N-[([1,1'-biphenyl]-4-yl)sulfonyl]-N-({1-[3,4,6-tri-O-acetyl-2-(acetylamino)-2-deoxy-beta-D-glucopyranosyl]-1H-1,2,3-triazol-4-yl}methyl)-D-valine | C34 H41 N5 O12 S | 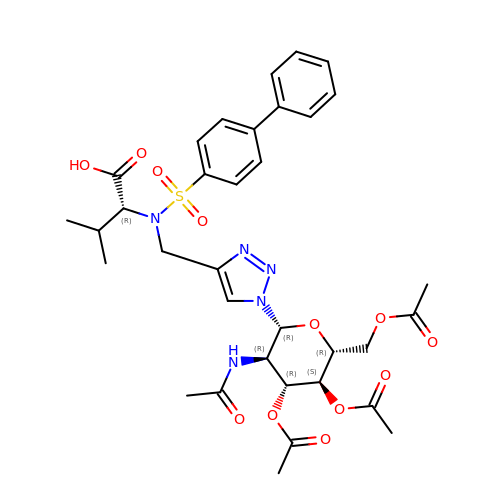GSNSTVUMMDDHHK-LNEPMPHRSA-N>MLITDTLSPQAFEEALRAKGDFYHIHHPYHIAMHNGNATREQIQGWVANRFYYQTTIPLKDAAIMANCPDAQTRRKWVQRILDHDGSHGEDGGIEAWLRLGEAVGLSRDDLLSERHVLPGVRFAVDAYLNFARRACWQEAACSSLTELFAPQIHQSRLDSWPQHYPWIKEEGYFFFR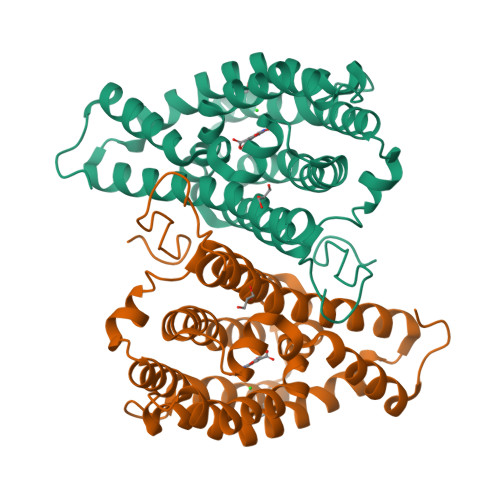SRLSQANRDVEHGLALAKAYCDSAEKQNRMLEILQFKLDILWSMLDAMTMAYALQRPPYHTVTDKAAWHTTRLVLEHHHHH[2x]Aerolysin is a β-pore-forming toxin produced by most Aeromonas bacteria, which has attracted large attention in the field of nanopore sensing due to its narrow and charged pore lumen. Pore-forming toxins (PFTs) are important virulence factors of many pathogenic bacteria, which are secreted in a soluble form and upon host membrane binding, they oligomerize into transmembrane pores undergoing a complex structural reorganization. Domains 3 and 4 form the 120 Å long 14-stranded β-barrel, with each protomer contributing two antiparallel β-strands. Four distinct constriction rings, two at each end of the pore, were identified from the structures and confirmed by MD simulation.

We obtained near-atomic resolution (2.2 Å) cryo-EM maps of WT aerolysin solubilized in either amphipols or SMALP, as well as in LMNG-CHS (2.6 Å). The cryoEM map in SMALPs shows an additional density, not observed with amphipol, which allows to partially model some of the lipids surrounding the β-barrel. Additional density is observed in the transmembrane part of the β-barrel in the SMALP data set which cannot be observed in the amphipol data set. This extra density allows one to partially fit some phospholipids and allows one to pinpoint the position of the aromatic belt formed by Y233 and W265 (YW belt) with respect to the membrane. Interestingly, just below the YW belt, two polar residues, E237 on one β-strand and Q263 on the opposite strand, interact with each other and are fully embedded at the core of the membrane hydrophobic environment. The high resolution of our structures allowed us to define a strong interaction of E237 with Q263 which is highlighted by the continuous density between the two residues. Carefully looking at the fitted model, such conformation could only be consistent with the formation of a double H-bond produced by a protonated E237, which is consistent with the expected higher pKa of glutamates within the hydrophobic environment of the membrane. In amphipol, K242 interacts with S256, while E254 interacts with K244; in the SMALP structure, K242 forms a salt-bridge with E254. The overall Cα root-mean-square deviation (RMSD) between the structures in amphipol and SMALP is 0.82 Å for the overall structures and 0.74 Å for the extended β-barrels region (i.e., residues 215–285).

>AEPVYPDQLRLFSLGQGVCGDKYRPVNREEAQSVKSNIVGMMGQWQISGLANGWVIMGPGYNGEIKPGTASNTWCYPTNPVTGEIPTLSALDIPDGDEVDVQWRLVHDSANFIKPTSYLAHYLGYAWVGGNHSQYVGEDMDVTRDGDGWVIRGNNDGGCDGYRCGDKTAIKVSNFAYNLDPDSFKHGDVTQSDRQLVKTVVGWAVNDSDTPQSGYDVTLRYDTATNWSKTNTYGLSEKVTTKNKFKWPLVGETELSIEIAANQSWASQNGGSTTTSLSQSVRPTVPARSKIPVKIELYKADISYPYEFKADVSYDLTLSGFLRWGGNAWYTHPDNRPNWNHTFVIGPYKDKASSIRYQWDKRYIPGEVKWWDWNWTIQQNGLSTMQNNLARVLRPVRAGITGDFSAESQFAGNIEIGAPVPLAA[7x]PTase is the key enzyme of the mannose 6-phosphate (M6P) targeting system that is responsible for tagging lysosomal hydrolases with the M6P moiety for their delivery to the lysosome. First, GlcNAc-1-phosphotransferase (PTase) transfers GlcNAc-1-phosphate (GlcNAc-1-P) from UDP-GlcNAc to mannose residues on the high mannose glycans of the hydrolases, following which the GlcNAc moiety is removed by uncovering enzyme to generate the M6P monoester. PTase is an α2β2γ2 heterohexamer encoded by two genes, GNPTAB and GNPTG. The α and β subunits are transcribed and translated from the GNPTAB gene as a precursor molecule that is cleaved by site-1 protease (S1P) at Lys-928 to generate the individual subunits, a critical step for the activation of the molecule.

Replacing S1 (233 aa) with a 29 aa linker sequence corresponding to the S1 region of the Dictyostelium discoideum PTase and deleting a large region from Notch 1 (N1) to the S1P cleavage site allowed for shortening of hPTase by 680 aa. The structure of soluble S1S3 was determined by single-particle cryo-EM at an overall resolution of 3.4 Å. Both 2D class averages and 3D maps show that S1S3 dimerizes similarly to PTase and has quite similar structural features as the catalytic core of PTase. The S1S3 structure comprises an NTE motif of two short α-helices, a large catalytic domain (the stealth domain) formed by the four conserved regions with a Rossmann-like GT-A fold, and a C-terminal small helix-bundle domain consisting of the EF hand and the three-helix S4 domain. Moreover, the EF hand interacts with CR4 of its counterpart subunit, thereby contributing to dimer formation. This finding explains why mutations within the EF-hand cause disease and inactivate the protein. S1S3 superimposes well on hPTase and zebrafish PTase (zPTase) with an RMSD of 0.63 and 0.75, respectively. S1S3 has essentially the same catalytic pocket with the catalytic NDD motif in the same orientation as other PTase structures. However, while hPTase fluctuates between an active and inactive state due to an auto-inhibitory motif that moves in and out of the catalytic pocket corresponding with the closed and open nature of the S1 domain, S1S3 lacks both the S1 domain and the region from N1 to the S1P cleavage site that contains the auto-inhibitory motif. Thus, S1S3 is likely locked in a constitutively active open state, consistent with its kinetic parameters.

>[2x]DEDQVDPRLIDGKWSRDQYHVLFDSYRDNIAGKSFQNRLCLPMPIDVVYTWVNGTDLELLKELTELKRSKRDPLIPECQGKQTPEKDKCYRDDISASRFEDNEELRYSLRSIERHAPWVRNIFIVTNGQIPSWLNLDNPRVTIVTHQDVFRNLSHLPTFSSPAIESHIHRIEGLSQKFIYLNDDVMFGKDVWPDDFYSHSKGQKVYLTWPVPNGGSGGDTFADSLRYVNKILNSKFGFTSRKVPAHMPHMIDRIVMQELQDMFPEEFDKTSFHKVRHSEDMQFAFSYFYYLMSAVQPLNISQVFDEVDTDQSGVLSDREIRTLATRIHELPLSLQDLTGLEHMLINCSKMLPADITQLNNIPPTQESYYDPNLPPVTKSLVTNCKPVTDKIHKAYKDKNKYRFEIMGEEEIAFKMIRTNVSHVVGQLDDIRKNPRKFVCLNDNIDHNHKDAQTVKAVLRDFYESMFPIPSQFELPREYRNRFLHMHELQEWRAYRDKLK>[2x]AGGQLNEFSSSGLGRAYSGEGAIADDAGNVSRNPALITMFDR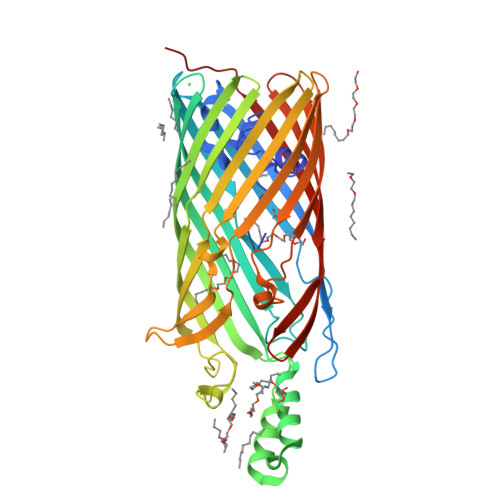PTFSAGAVYIDPDVNISGTSPSGRSLKADNIAPTAWVPNMHFVAPINDQFGWGASITSNYGLATEFNDTYAGGSVGGTTDLETMNLNLSGAYRLNNAWSFGLGFNAVYARAKIERFAGDLGQLVAGQIMQSPAGQTQQGQALAATANGIDSNTKIAHLNGNQWGFGWNAGILYELDKNNRYALTYRSEVKIDFKGNYSSDLNRAFNNYGLPIPTATGGATQSGYLTLNLPEMWEVSGYNRVDPQWAIHYSLAYTSWSQFQQLKATSTSGDTLFQKHEGFKDAYRIALGTTYYYDDNWTFRTGIAFDDSPVPAQNRSISIPDQDRFWLSAGTTYAFNKDASVDVGVSYMHGQSVKINEGPYQFESEGKAWLFGTNFNYAFHHHHHH> MGPSFNPVRFLELPIDIRKEVYFHLDGNFCGAHPYPIDILYKSNDVELPGKPSYKRSKRSKKLLRYMYPVFATYLNIFEYSPQLIEKWLEYAFWLRYD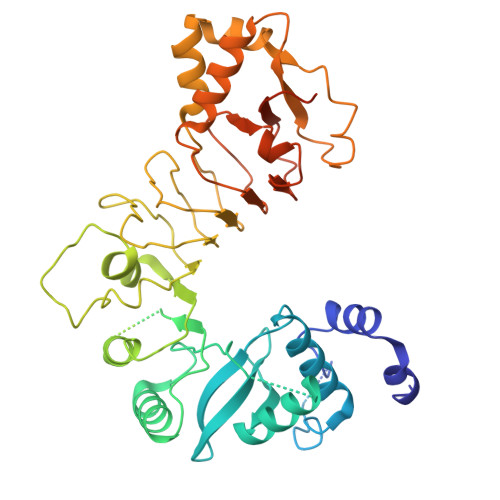CLVLDCFKVNHLYDGTLIDALEWTYLDNELRLAYFNKASMLEVWYTFKEYKKWVIDSVAFDELDLLNVSNIQFNIDNLTPQLVDKCLSILEQKDLFATIGEVQFGQDEEVGEEKDVDVSGANSDENSSPSSTIKNKKRSASKRSHSDNGNVGATHNQLTSISVIRTIRSMESMKSLRKITVRGEKLYELLINFHGFRDNPGKTISYIVKRRINEIRLSRMNQISRTGLADFTRWDNLQKLVLSRVAYIDLNSIVFPKNFKSLTMKRVSKIKWWNIEENILKELKVDKRTFKSLYIKEDDSKFTKFFNLRHTRIKELDKSEINQITYLRCQAIVWLSFRTLNHIKLQNVSEVFNNIIVPRALFDSKRVEIYRCEKISQVLVIGSRSGSENLYFQGSKRRWKKNFIAVSAANRFKKISSSGAL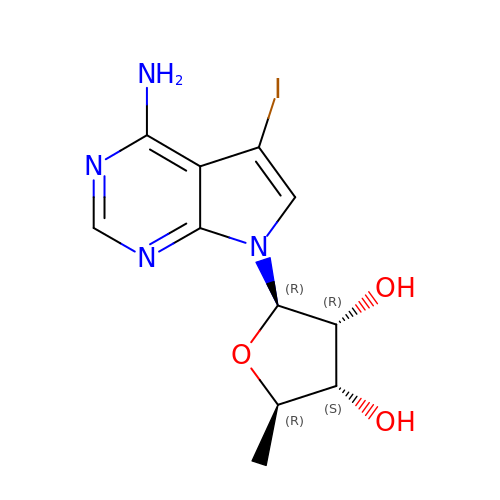7-(5-DEOXY-BETA-D-RIBOFURANOSYL)-5-IODO-7H-PYRROLO[2,3-D]PYRIMIDIN-4-AMINE | C11 H13 I N4 O3 | NTXUAWGNGBSCRS-TZQXKBMNSA-N(2~{S},3~{S},4~{S},5~{R},6~{R})-6-[[(3~{S},4~{a}~{R},6~{a}~{R},6~{b}~{S},8~{a}~{S},11~{S},12~{a}~{R},14~{a}~{R},14~{b}~{S})-11-carboxy-4,4,6~{a},6~{b},8~{a},11,14~{b}-heptamethyl-14-oxidanylidene-2,3,4~{a},5,6,7,8,9,10,12,12~{a},14~{a}-dodecahydro-1~{H}-picen-3-yl]oxy]-3,4,5-tris(oxidanyl)oxane-2-carboxylic 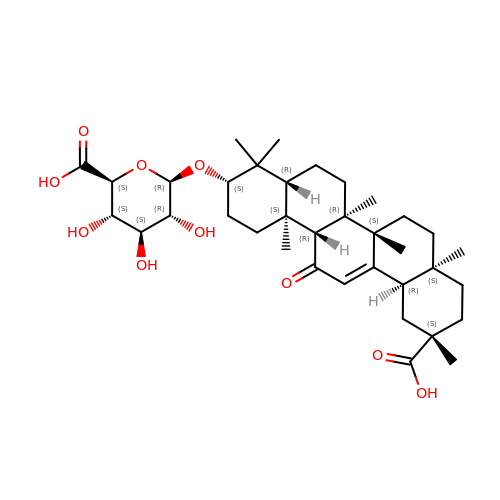acid | C36 H54 O10 | HLDYLAJAWSKPFZ-QDPIGISRSA-N> GMRRQTMVKAGAVACAVALLGSLSACGGSKKSTTTADGKPI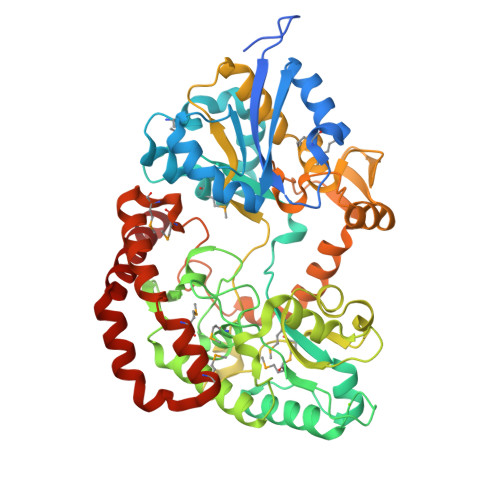VTVLVKKNANQEKMANMQWAKDLEADCDCKIEWQEVTREAWAQQKNATLASGDIADVNLNGYGAVEAYQYPGMFEDLSKDLDKLPNVKAFFKQKPDAKKMSTDSKGRIYAIADGRGKAYSGTGQHMLINKAWLDKLGLQVPTTWDELENVLKAFKTQDPNGNGQADEIPMNIKKLEGSYFTWYSPMLLLNSTGIVTGFNKGVSEYGFYAKNGVVKSFLTSDEYKEVIKYYHKLISEGLIPAEWATKDDDAYNADQISDGKTAKTGVVFGWSPSDNFGKLKDQYIAMPVPSAPGVSPDQTVWDGSSSELSPAGLSISSHAANKDAALKLANLLYSEKYSVQQFLGSFGKAITKTGEHEYTVDNDKLSQLTGDNQYPGLSELLVGWIPDEATIKGDTHADELIEVNKVYEEQRSHFDPVKDYIPDYVNMDNMDPSDATKLNTNNAEIFNTTMQKTATWMSKGGIDEEWDAYCKQLDSIGLQESTKIWQKWYDTYTK> MWNPIVNVDITLNTAGTTREGFGLPLFLASTDNFEERIRGYTSLTEVAEDFDESTAAYKAAKQLWSQTPKVTQLYIGRRTMQYTVSIPDTVAEGSEYSLTVAIGGGVSQPFQYTAKENDTALIVLNEFKSQIEASPTIKDGVNASVTGTGASAT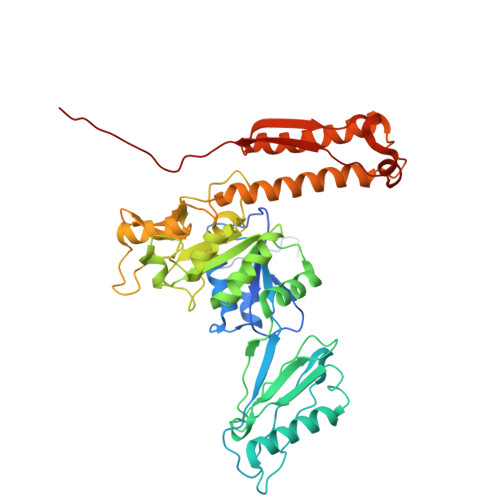MIITKAGDNDFVKVTSITPTTSIAATTADTASAALASIETYSTDWYFISAEDRTQQFVLAMASEIQARKKIFFTANADVKALQGTDLTSATDVPAQLAKSKYTRTVCLWHHTAEFDYPEMAYIAYGAPYDAGSIAWGNAQLTGVAASLQPANQRPLISIQKSALDTRSCNFIDLDGGVPVVRRGITSGGEWIDIVRGVDWLESDLKTSLRDLLINQKGGKITYDDTGITRIRQVIETSLQRAVNRKFLSTYTVTVPKASQVALADKKARILKDITFHGILAGAILDVDLKGTVAYE> MHHHHHHAVRASEISRVYEAYPEKKATLY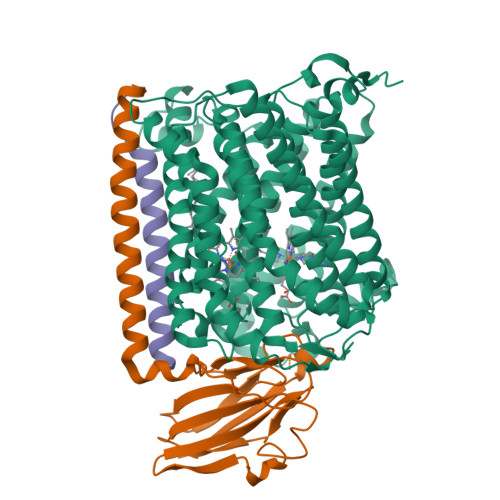FLVLGFLALIVGSLFGPFQALNYGNVDAYPLLKRLLPFVQSYYQGLTLHGVLNAIVFTQLFAQAIMVYLPARELNMRPNMGLMWLSWWMAFIGLVVAALPLLANEATVLYTFYPPLKGHWAFYLGASVFVLSTWVSIYIVLDLWRRWKAANPGKVTPLVTYMAVVFWLMWFLASLGLVLEAVLFLLPWSFGLVEGVDPLVARTLFWWTGHPIVYFWLLPAYAIIYTILPKQAGGRLVSDPMARLAFLLFLLLSTPVGFHHQFADPGIDPTWKMIHSVLTLFVAVPSLMTAFTVAASLEFAGRLRGGRGLFGWIRALPWDNPAFVAPVLGLLGFIPGGAGGIVNASFTLDYVVHNTAWVPGHFHLQVASLVTLTAMGSLYWLLPNLTGKPISDAQRRLGLAVVWLWFLGMMIMAVGLHWAGLLNVPRRAYIAQVPDAYPHAAVPMVFNVLAGIVLLVALLLFIYGLFSVLLSRERKPELAEAPLPFAEVISGPEDRRLVLAMDRIGFWFAVAAILVVLAYGPTLVQLFGHLNPVPGWRLW;> MVDQHKAHKAILAYEKGWLAFSLAMLFVFIALIAYTLATHTAGVIPAGKLERVDPTTVRQEGPWADPAQAVVQTGPNQYTVYVLAFAFGYQPNPIEVPQGAEIVFKITSPDVIHGFHVEGTNINVEVLPGEVSTVRYTFKRPGEYRIICNQYCGLGHQNMFGTIVVKE;> MEEKPKGALAVILVLTLTILVFWLGVYAVFFARG The pyridoxal 5′‐phosphate (PLP) homeostasis protein (PLPHP) is a ubiquitous member of the COG0325 family with apparently no catalytic activity. Although the actual cellular role of this protein is unknown, it has been observed that mutations of the PLPHP encoding gene affect the activity of PLP‐dependent enzymes, B6 vitamers and amino acid levels. Here we report a detailed characterization of the Escherichia coli ortholog of PLPHP (YggS) with respect to its PLP binding and transfer properties, stability, and structure. YggS binds PLP very tightly and is able to slowly transfer it to a model PLP‐dependent enzyme, serine hydroxymethyltransferase.

We serendipitously discovered that the K36A variant of YggS, affecting the lysine residue that binds PLP at the active site, is able to bind PLP covalently. This observation led us to recognize that a number of lysine residues, located at the entrance of the active site, can replace Lys36 in its PLP binding role.

> MNDIAHNLAQVRDKISAAATRCGRSPEEITLLAVSATAPASAIAEAIDAGQRQFGENYVQEGVDKIRHFQELGVTGLEWHFIGPLQSNKSRLVAEHFDWCHTIDRLRIATRLNDQRPAELPPLNVLIQINISDENSKSGIQLAELDELAAAVAELPRLRLRGLMAIPAPESEYVRQFEVARQMAVAFAGLKTRYPHIDTLSLGMSDDMEAAIAAGSTMVRIGTAIFGARDYSAA> GAGGAGCCTGCGCGGACAGAG;> CCGCGCA;> GGCTCC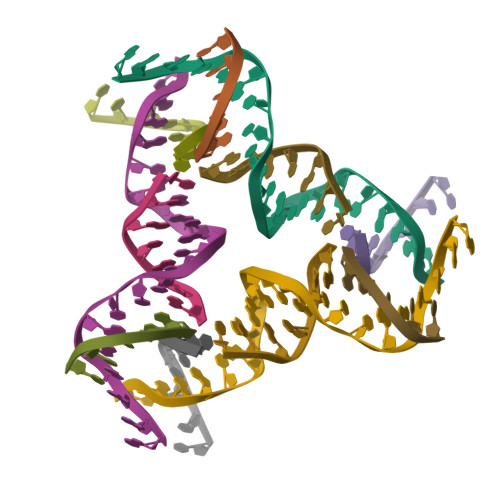;> TCCTCTGT> SPTPLPQLPSNVRDGENNVASTFLQAFFQLWDHDRLTLIPQFYDSETTFSVVFATDSPQDPASSSCSKFSRNLNILSPRHPSTLQRLFVGSNLIADLWKVLPATRHPSLDQTSQWLIDCHTFPHLADPTGMAPYAMGLMINVNGQCEEADISQNLYGTRTFSRCFILGPSKPGAPHPYRVLSDQLTLHTWKPQ;> MLSRRYAAKSFVEWYYRQINENKPVASGYVNNNATYTKAGHPPADITINGRVVATPEEWDTMLKEQRAQHNTSSSSTLPIGRKPVRYDVDCFDVHVINADYRFAAPQRMIEQHAPTDGVRMMMALTVSGSVYFGASP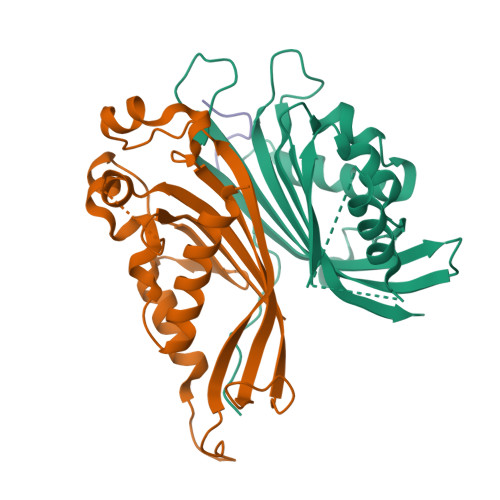RSTDDYVIKQHFNDVFILVPNWDVLEKPGARSGRKYLIASHKYRAY;> FASPAPSNQGSSVFGAPAQST ISOVALERIC ACID | C5 H10 O2 | 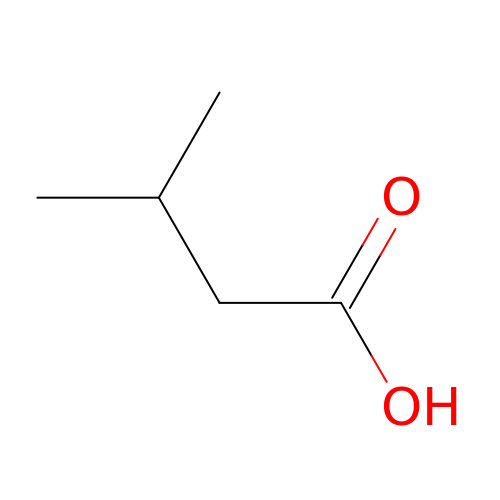GWYFCOCPABKNJV-UHFFFAOYSA-N> LTDLTKNEKGRLTPITKQQSANSAKLTAYGTLKSALEKFQTANTALNKADLFKSTVA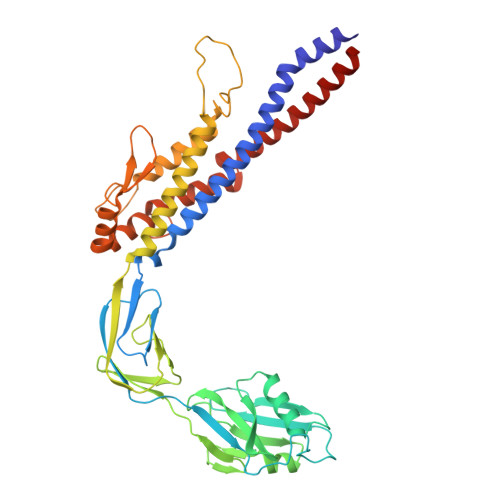SSTTEDLKVSTTAGAAAGTYKINVTQLAAAQSLATKTTFATTKEQLGDTSVTSRTIKIEQPGRKEPLEIKLDKGDTSMEAIRDAINDADSGIAASIVKVKENEFQLVLTANSGTDNTMKITVEGDTKLNDLLAYDSTTNTGNMQELVKAENAKLNVNGIDIERQSNTVTDAPQGITLTLTKKVTDATVTVTKDDTKAKEAIKSWVDAYNSLVDTFSSLTKYTAVEPGEEASDKNGALLGDSVVRTIQTGIRAQFANSGSNSAFKTMAEIGITQDGTSGKLKIDDDKLTKVLKDNTAAARELLVGDGKETGITTKIATEVKSYLADDGIIDNAQDNVNATLKSLTKQYLSVSNSIDETV>STPFGLDLGNNNSVLAVARNRGIDIVVNEVSNRSTPSVVGFGPKNRYLGETGKNKQTSNIKNTVANLKRIIGLDYHHPDFEQESKHFTSKLVELDDKKTGAEVRFAGEKHVFSATQLAAMFIDKVKDTVKQDTKANITDVCIAVPPWYTEEQRYNIADAARIAGLNPVRIVNDVTAAGVSYGIFKTDLPEGEEKPRIVAFVDIGHSSYTCSIMAFKKGQLKVLGTACDKHFGGRDFDLAITEHFADEFKTKYKIDIRENPKAYNRILTAAEKLKKVLSANTNAPFSVESVMNDVDVSSQLSREELEELVKPLLERVTEPVTKALAQAKLSAEEVDFVEIIGGTTRIPTLKQSISEAFGKPLSTTLNQDEAIAKGAAFICAIHSPTLRVRPFKFEDIHPYSVSY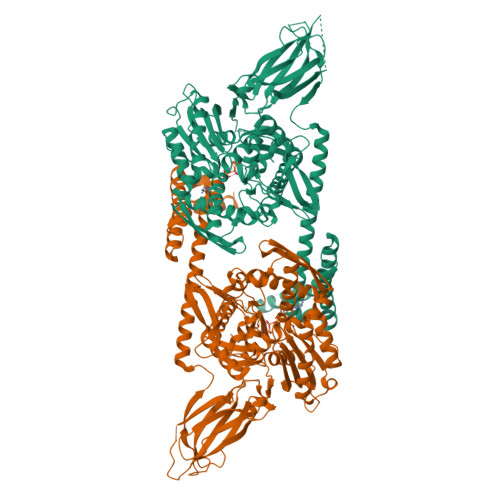SWDKQVEDEDHMEVFPAGSSFPSTKLITLNRTGDFSMAASYTDITQLPPNTPEQIANWEITGVQLPEGQDSVPVKLKLRCDPSGLHTIEEAYTIEDIEVEEPIPLPEDAPEDAEQEFKKVTKTVKKDDLTIVAHTFGLDAKKLNELIEKENEMLAQDKLVAETEDRKNTLEEYIYTLRGKLEEEYAPFASDAEKTKLQGMLNKAEEWLYDEGFDSIKAKYIAKYEELASLGNIIRGRYLAKEEEKKQAIRSKQEA[2x]The ClpP protease is found in all kingdoms of life, from bacteria to humans. Here we show that, in contrast to this general architecture, the Clp protease from Mycobacterium smegmatis (Msm) forms an asymmetric hetero-oligomeric complex ClpP1P2, which only associates with its cognate ATPase through the ClpP2 ring. Our structural and functional characterisation of this complex demonstrates that asymmetric docking of the ATPase component is controlled by both the composition of the ClpP1 hydrophobic pocket (Hp) and the presence of a unique C-terminal extension in ClpP1 that guards this Hp. The catalytic residues (Ser-His-Asp), of this complex, are encapsulated within the barrel-shaped proteolytic chamber and access to the chamber is restricted to a narrow entry portal at either end of the complex.

The structure of MsmClpP1 was determined to 2.0 Å resolution and refined to an Rfree value of 21.5%. Similar to other ClpP structures, MsmClpP1 was composed of two heptameric rings stacked back-to-back (the asymmetric unit consisted of one heptamer, the biological tetradecamer is formed from crystallographically related heptamers). The tetradecamer forms a compact barrel-shaped oligomer with approximate dimensions 86 × 102 Å. Compared to these active structures, both MsmClpP1 and MtbClpP1, have shorter handle domains, which lack a structured β-strand region. As a result, association of the heptameric rings in MsmClpP1 (and MtbClpP1) is mediated largely by a trans association of a short section of the α-helix in the handle domain creating several openings in the side-walls of the ClpP1 tetradecamer. Significantly, the breaches in the side wall of MsmClpP1 are located adjacent to the catalytic residues of the protease and as such provide a direct path between the active site of the protease and the external solution. Hence as has been proposed by Kay and Houry33, these openings could represent an exit portal for the egress of peptides. Therefore, we postulate that this structure of MsmClpP1 represents a post “substrate-cleavage” snapshot of the protease. Another distinctive feature of MsmClpP1, which is absent in many ClpP homologues including MtbClpP124,32, is a short C-terminal extension (CTE) ~12 residues long, which docks into its own Hp. Specifically, the CTE interacts with three tyrosine residues (Y60, Y88 and Y110) within the Hp.

>MTDMRGTGQGLNLVDSVYERLLAERIIFLGSQVDDDIANRLCAQILLLSAEDPTKDIHLYINSPGGSISAGMAIYDTMVLAPCDIATYAMGMAASMGEFLLAAGTKGKRYALPHARILMHQPLGGVTGSAADIAIQAEQFAVIKKEMFRLNAEFTGQPIERIEADSDRDRWFTAQEALEYGFVDHIITSASVNGEGPGAGLDKAAAHHHHHHHHHH[7x]> MFESMKPHLAELRQRLAISVLAVFVGFIIAFTFHNAILGWITKPLNNALIQVGKIVEKREMGTWKISGNEHNATLAPSKSPALLSDHAQSAEKLHRTLAEASQATQNPKLQKLLSQAASAAEELARNSRILRKALVKEENLTRQAVNQNLREKSFNGMITTHQVGGAFFVALKVSFFAGILMAMPVILWQLWLFIAPGLYDNEKKMVLPFVVGGSVMFLIGVLFAYYVVTPFGFQFLITFGSFLYTPLINIEDYVGFFTKILIG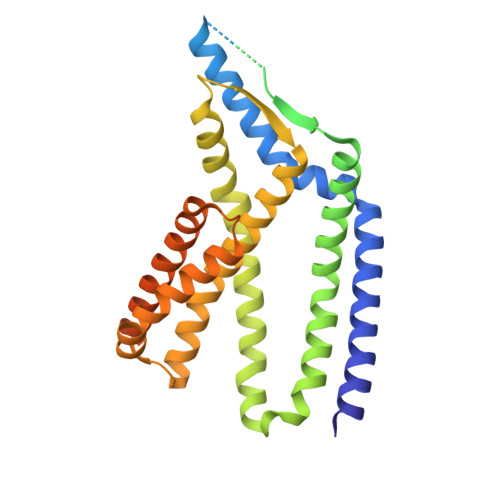FGIAFELPVVAYFLALLGLITDKTLKDYFKYAIVIIFLLAAFLTPPDVLTQLLMAAPLILLYGLSILIVHYVNPYKPEEKEDDEEEEEDEFEKAEREFEALEKGSESHESGSENLYFQ> GEKKECWSWESYLEEQKAITAPVSLFQDSQAVTHNKNGFKLGMKLEGIDPQHPSMYFILTVAEVCGYRLRLHFD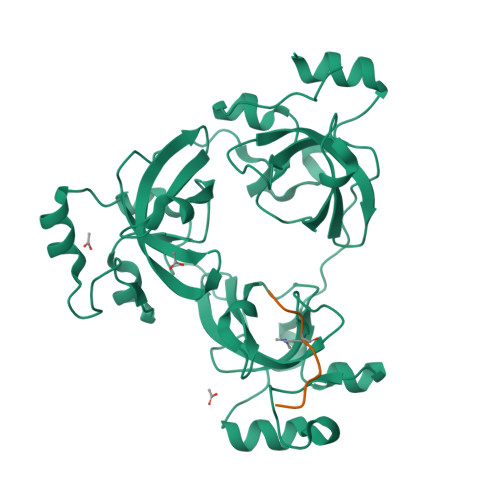GYSECHDFWVNANSPDIHPAGWFEKTGHKLQPPKGYKEEEFSWSQYLRSTRAQAAPKHLFVSQSHSPPPLGFQVGMKLEAVDRMNPSLVCVASVTDVVDSRFLVHFDNWDDTYDYWCDPSSPYIHPVGWCQKQGKPLTPPQDYPDPDNFCWEKYLEETGASAVPTWAFKVRPPHSFLVNMKLEAVDRRNPALIRVASVEDVEDHRIKIHFDGWSHGYDFWIDADHPDIHPAGWCSKTGHPLQPPLGPRE;> RHRKVLRDN CYCLOPENTYL 2-OXO-4-PHENYLAZETIDINE-1-CARBOXYLATE 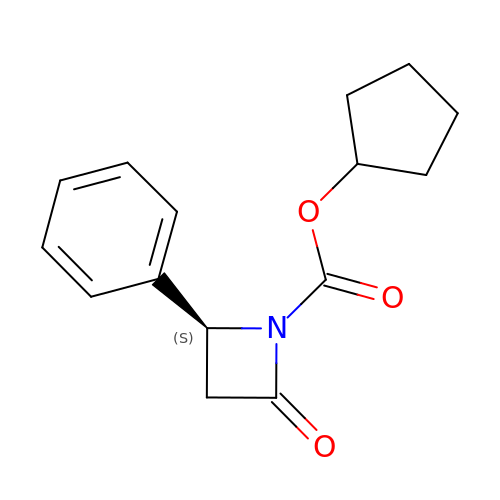| C15 H17 N O3 | HXGULOODWVYRBT-ZDUSSCGKSA-N> MTQMRFTEEDFNTFTIEGLDARMEVLKETVRPKLTALGEHFAPTLSALTGDEMFPHVAKHARRSVNPPADSWVAFANSKRGYKKLPHFQIGLWESHVFVWFAIIYESPIKEEYGKLLEVNQET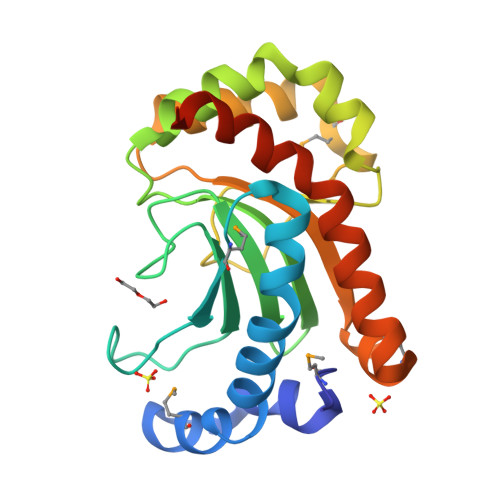ITKNIPDSFVWSADHTKPGVHKQSEMDKEQLKTLFERLQTVKKAELLCGIQLQKEEVLNMNNQEFLQRIDDAFKQLAFLYRLTQKVTQALEHHHHHH> PEDPSDLLQHVKFQSSNFENILTWDSGPEGTPDTVYSIEYKTYGERDWVAKKGCQRITRKSCNLTVETGNLTELYYARVTAVSAGGRSATKMTDRFSSLQHTTLKPPDVTCISKVRSIQMIVHPTPTPIRAGDGHRLT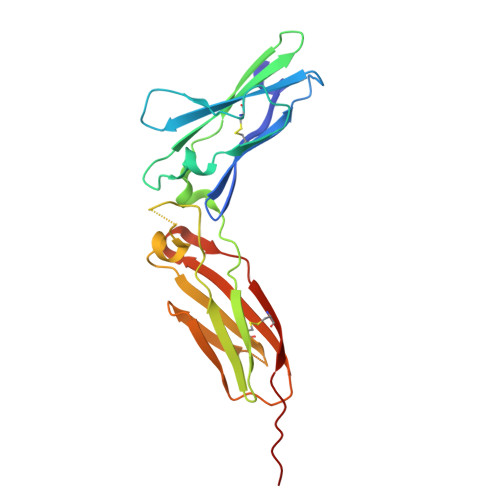LEDIFHDLFYHLELQVNRTYQMHLGGKQREYEFFGLTPDTEFLGTIMILVPTWAKESAPYMCRVKTLPDRTWT>[2x]MIVSDIEANALLESVTKFHCGVIYDYSTAEYVSYRPSDFGAYLDALEAEVARGGLIVFHNGHKYDVPALTKLAKLQLNREFHLPRENCIDTLVLSRLIHSNLKDTDMGLLRSGKLPGALEAWGYRLGEMKGEYKDDFKRMLEEQGEEYVDGMEWWNFNEEMMDYNVQDVVVTKALLEKLLSDKHYFPPEIDFTDVGYTTFWSESLEAVDIEHRAAWLLAKQERNGFPFDTKAIEELYVELAARRSELLRKLTETFGSWYQPKGGTEMFCHPRTGKPLPKYPRIKTPKVGGIFKKPKNKAQREGREPCELDTREYVAGAPYTPVEHVVFNPSSRDHIQKKLQEAGWVPTKY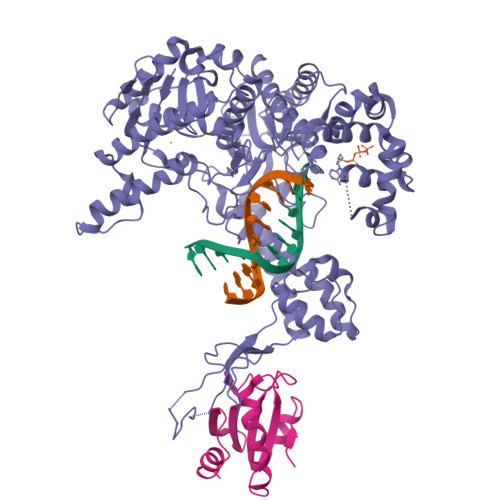TDKGAPVVDDEVLEGVRVDDPEKQAAIDLIKEYLMIQKRIGQSAEGDKAWLRYVAEDGKIHGSVNPNGAVTGRATHAFPNLAQIPGVRSPYGEQCRAAFGAEHHLDGITGKPWVQAGIDASGLELRCLAHFMARFDNGEYAHEILNGDIHTKNQIAAELPTRDNAKTFIYGFLYGAGDEKIGQIVGAGKERGKELKKKFLENTPAIAALRESIQQTLVESSQWVAGEQQVKWKRRWIKGLDGRKVHVRSPHAALNTLLQSAGALICKLWIIKTEEMLVEKGLKHGWDGDFAYMAWVHDEIQVGCRTEEIAQVVIETAQEAMRWVGDHWNFRCLLDTEGKMGPNWAICH;>SDKIIHLTDDSFDTDVLKADGAILVDFWAEWCGPCKMIAPILDEIADEYQGKLTVAKLNIDQNPGTAPKYGIRGIPTLLLFKNGEVAATKVGALSKGQLKEFLDANLA[2x]> NGDRLYRADSRPPDEIKRSGGLMPRGHNEYFDRGTQMNICLYDHARGTQTGFVRYDDGYVSTSLSLRSAHLAGQSILSGYSTYYIYVIATAPNMFNVNDVLGVYSPHPYEQEVSALGGIPYSQIYGWYRVNFGVIDERL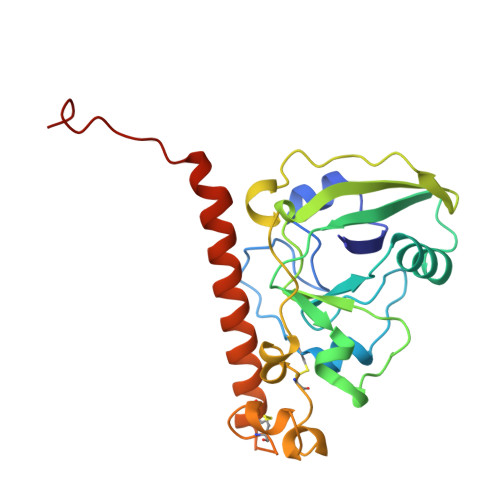HRNREYRDRYYRNLNIAPAEDGYRLACFPPDHQAWREEPWIHHAPQGCGNSSRTITGDTCNEETQNLSTIYLREYQSKVKRQIFSDYQSEVDIYNRIRDEL> QDWLTFQKKHITNTRD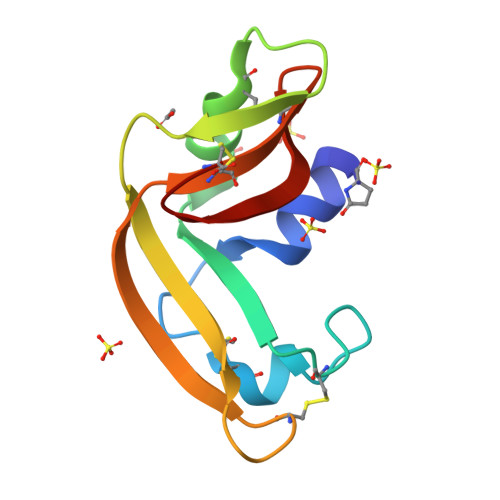VDCDNIMSTNLFHCKDKNTFIYSRPEPVKAICKGIIASKNVLTTSEFYLSDCNVTSRPCKYKLKKSTNKFCVTCENQAPVHFVGVGSC>[4x]MNAESRYVLTGRYDSAPATDGSGTALGWTVAWKNNYRNAHSATTWSGQYVGGAEARINTQWLLTSGTTEANAWKSTLVGHDTFTKVKPSAASGGGSAEA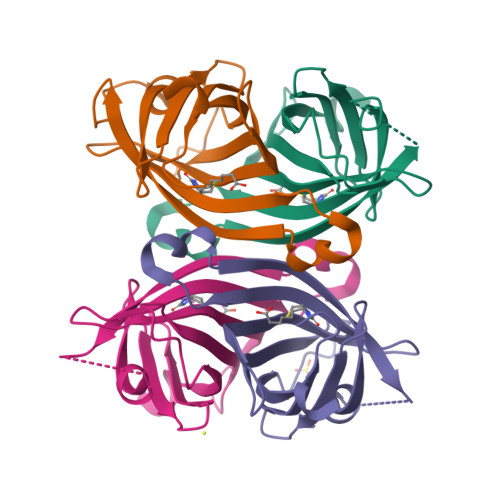GITGTWYNQLGSTFIVTAGADGALTGTYESAVG>[4x]MHHHHHHMTMDEQQPQAVTPVYVGGF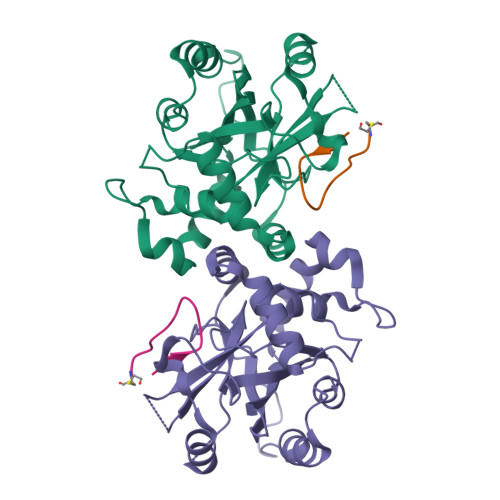LARYDQSPDEAELLLPRDVVEHWLHAQGQGQPSLSVALPLNINHDDTAVVGHVAAMQSVRDGLFCLGCVTSPRFLEIVRRASEKSELVSRGPVSPLQPDKVVEFLSGSYAGLSLSSRRCDDVEQATSLSGSETTPFKHVALCSVGRRRGTLAVYGRDPEWVTQRFPDLTAADRDGLRAQWQRCGSTAVDASGDPFRSDSYGLLGNSVDALYIRERLPKLRYDKQLVGVTERESYVKA;>FITGHYWVRFLPC[3x]(2S)-2-{[(2S)-2-{[(2S)-2-hydroxypropyl]oxy}propyl]oxy}propan-1-ol | C9 H20 O4 | 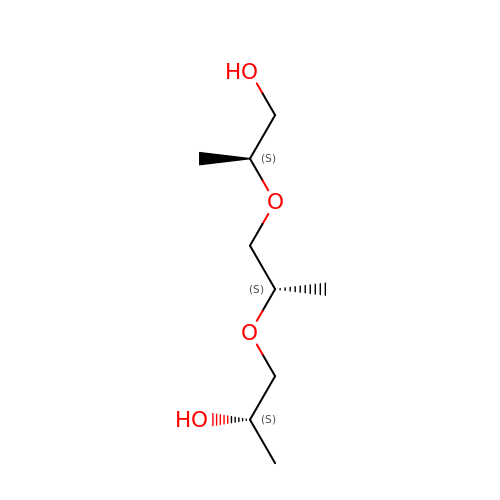LCZVSXRMYJUNFX-CIUDSAMLSA-N> APLAGGDGFSLHPPYFNLAEGARITASATCGEEAPTRSVSRPTEDLYCKLVGGPVAGGDPAQTIQGQYCDICTAANSNKAHPVSNAIDGTERWWQSPPLSRGLEYNEVNVTLDLGQVFHVAYVLIKFANSPRPDLWVLERSTDFGHTYQPWQFFASSKRDCLERFGPRTLERITQDDDVICTTEYSRIVPLENGEIVVSLVNGRPGALNFSYSPLLRDFTKATNIRLRFLRTNTLLGHLMGKALRDPTVTRRYYYSIKDISIGGRCVCHGHADVCDAKDPLDPFRLQCACQHNTCGGSCDRCCPGFNQQPWKPATTDSANECQSCNCHGHAYDCYYDPEVDRREASQNQDNVYQGGGVCLDCQHHTTG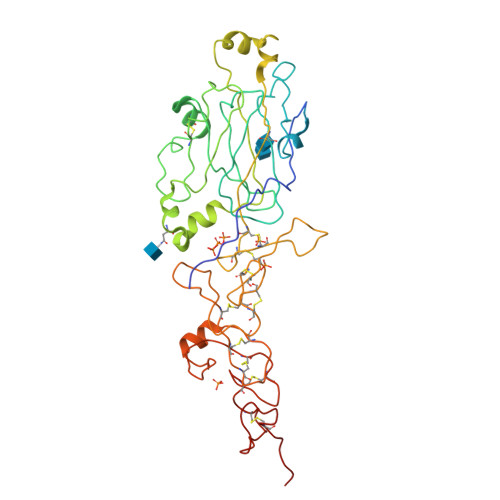INCERCLPGFFRAPDQPLDSPHVCRPAAAHHHHHH> MGSDKIHHHHHHENLYFQGMLFHQVFFWLKNPGDKADRDKLIAGLKALKAIDVIQQLHVGVPAATEKRDVVDNSYDVSELMVFKSVEDQKRYRDHPLLQKFVADCSHLWS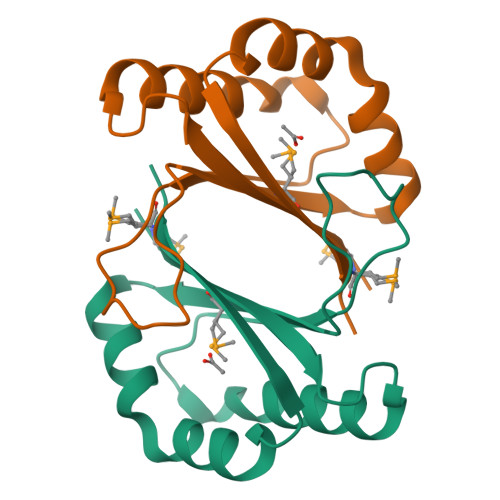KVVVYDSMSV>HHHHHHSSGLVPRGSHMTDLNIPHTHAHLVDAFQALGIRAGQALMLHASVKAVGAV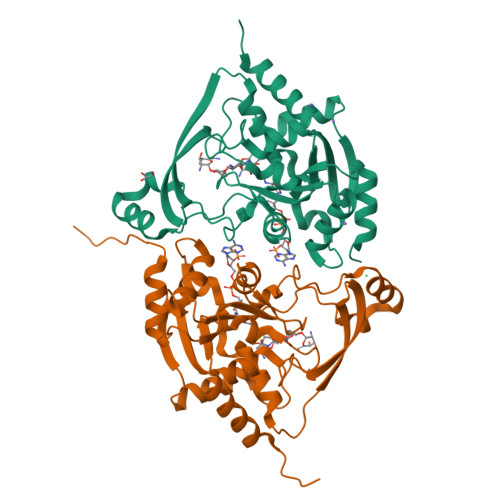MGGPNVILQALMDALTPDGTLMMYAGWQDIPDFIDSLPDALKAVYLEQHPPFDPATARAVRENSVLAEFLRTWPCVHRSANPEASMVAVGRQAALLTANHALDYGYGVESPLAKLVAIEGYVLMLGAPLDTITLLHHAEYLAKMRHKNVVRYPCPILRDGRKVWVTVEDYDTGDPHDDYSFEQIARDYVAQGGGTRGKVGDADAYLFAAQDLTRFAVQWLESRFGDSASYG[4x]>[2x]AYRDQPLGELALSIPRASALFRKYDMDYAAGGKQTLARAAARKELDVEVIEAELAKLAEQPIEKDWRSAPLAEIIDHIIVRYHDRHREQLPELILQATKVERVHADKPSVPKGLTKYLTMLHEELSSHMMKEEQILFPMIKQGMGSQAMGPISVMESLHDEAGELLEVIKHTTNNVTPPPEACTTWKAMYNGINELIDDLMDHISLENNVLFPRALAGE

Escherichia coli YtfE is a di-iron protein of the widespread Repair of Iron Centers proteins (RIC) family that has the capacity to donate iron, which is a crucial component of the biogenesis of the ubiquitous family of iron-sulfur proteins. Bacterial RICs are composed by an N-terminal ScdA-like domain and a C-terminal domain that folds as a four-helix bundle where a histidine/carboxylate di-iron type center is inserted. In E. coli YtfE, the best studied RIC protein, the center is coordinated by H84, H129, H160, H204, and two μ-carboxylate bridges formed by E133 and E208. We show that YtfE establishes protein-protein interactions with the scaffold IscU, where the transient cluster is formed, and the cysteine desulfurase IscS.

However, in YtfE-E159L with a neutral leucine instead of the glutamate, the metal site lost one of its iron ions. The structure of YtfEM-E159L contains only one iron atom in the metal center that is located ca. 13 Å below the channel entrance. In this case, the channel is longer, with a length of about 16 Å, and although the channel entrance retains the circular shape, its diameter is reduced to ∼1.5 Å. The channel is also formed by hydrophilic residues, namely by the ligands H204, H129, H160, and residues E125, E162, and L166 located at the channel entrance. In YtfEM-E159L, the absence of the second Fe atom, the different position of the H129 sidechain (mentioned above) and the presence of leucine in position 159 modified the channel arrangement so that the substituting L159 residue is no longer included in the channel. Additionally, the conformation of ligand H129 differs from that observed in the other two proteins. Specifically, the side chain of H129 is ∼7 Å apart from its original position and no longer pointing toward the di-iron center (the closest distance to YtfEM-E159L H129 is ca. 9 Å whereas in YtfeM it is about 2 Å). Moreover, the structure of YtfEM revealed that when E159, that establishes a hydrogen bond with the iron ligand H129 (H129Nδ1.E159Oε1-2.66 Å), is replaced by leucine, the position of the neighboring histidine H129 alters its sidechain conformation, pointing away from the center and toward the protein surface. Interestingly, in the YtfEM-E159L structure, no such hydrogen bond interactions are present, probably explaining why the B-values in this domain are higher than in the other structures. Thermodynamic and kinetic data indicate that mutation of E159 generates a protein with a more unstable center that releases iron at a higher rate. The mononuclear iron YtfE-E159L mimics an YtfE protein following iron release and its structure shows that the process implies the movement of one of the axial histidines that exposes the metal site cavity to the exterior, thus making possible the re-entry of another iron atom to rebuild the di-iron center.>[2x]MHHHHHHMTKQALLEVSNLVREFPAGESTIQILKGIDLTIYEGELVAIVGQSGSGKSTLMNILGCLDRPTSGSYKVNGQETGKLEPDQLAQLRREYFGFIFQRYHLLGDLSAEGNVEVPAVYAGVTPADRKQRATALLTELGLGTKTQNRPSQLSGGQQQRVSIARALMNGGDVILADEPTGALDSHSGVEVMRILRELNAAGHTIILVTHDMQVAKNATRIIEISDGEIISDRPNVPDQSLEEVKSDPDAAPALQNKQKKG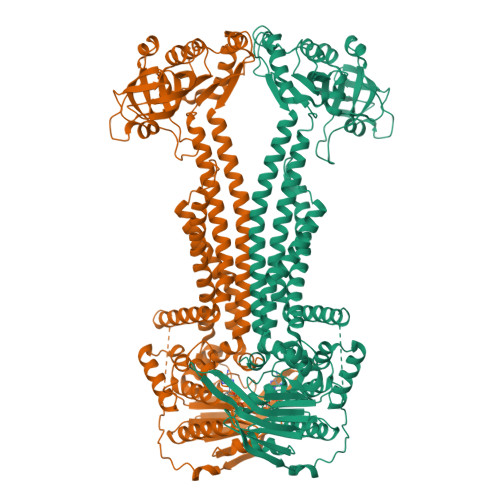KSISAWRSTLDRLSEAFQMALLSMNAHRMRTFLTMLGIIIGIASVVTVVALGNGSQQQILSNISSLGTNTITVFQGRGFGDNSKTANFKTLVPADADALMTQPYVSAVSPMVSTSKTMRYQQNEANATINGVSNDYFDVKGLVFKDGQTFDQRSVRDRSQDVVIDTNTQKQFFSDGTNPIGQVVLLGSVPARIIGIVEPQTSGMGSDDTLNVYMPYTTVMSRMLGQAHVRNIVVRINDKYSTSAAENAIVNLLTQRHGAQDIFTMNSDSIRQTIEKTTSTMTLLVSAIAVISLVVGGIGVMNIMLVSVTERTQEIGVRMAVGARQSDILQQFLIEAILVCLIGGVLGVLLSLGLGQLINKFAGGNFAVAYSTTSIVAAFVCSTLIGVVFGFLPAKNAAKLDPVAALSRE>[6x]MSNLPHEPEFEQAYKELASTLENSTLFQKNPEYRKALAVVSVPERVIQFRVVWEDDAGNVQVNRGFRVQFNSALGPYKGGLRFHPSVNLSILKFLGFEQIFKNALTGLNMGGGKGGSDFDPKGKSDNEIRRFCVSFMTELCKHIGADTDVPAGDIGVTGREVGFLFGQYRKIRNQWEGVLTGKGGSWGGSLIRPEATGYGVVYYVEHMIAHATNGQESF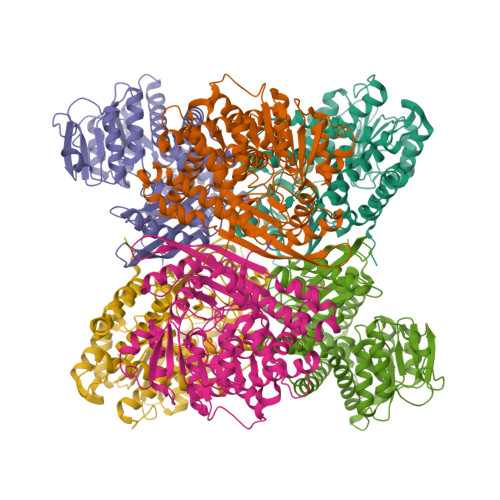KGKRVAISGSGNVAQYAALKVIELGGSVVSLSDSQGSLIINGEGSFTPEEIELIAQTKVERKQLASIVGAAPFSDANKFKYIAGARPWVHVGKVDVALPSATQNEISGEEAQVLINAGCKFIAEGSNMGCTQEAIDTFEAHRTANAGAAAIWYAPGKAANAGGVAVSGLEMAQNSARLSWTSEEVDARLKDIMRDCFKNGLETAQEYATPAEGVLPSLVTGSNIAGFTKVAAAMKDQGDWW> MDNKPETSLDNPVHQRSEPGSETGSSLSTITTHHLTVPPGLTPEEFQELSSSIAEFHSYRINPGQCSSLLAQRIHAPVETVWTVVRRFDKPQTYKHFIKSCSVGEDFRMTVGSTRDVTVISGLPAATSTERLDILDDDRHVTGFSIIGGDHRLRNYRSVTTVHGFERDGEIWTVVLESYVVDVPEGNTEE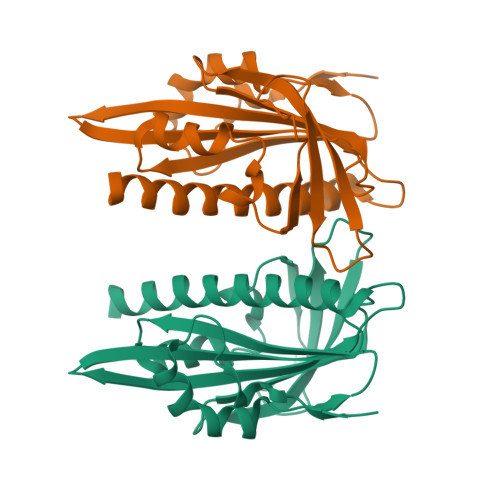DTRLFADTVVKLNLQKLASVTETLAREAGNGSVNSRDASHRS> MTHHHHHHAMALTDRGMTYDLDPKDGSSAATKPVLEVTKKVFDTAADAAGQTVTVEFKVSGAEGKYATTGYHIYWDERLEVVATKTGAYAKKGAALEDSSLAKAENNGNGVFVAS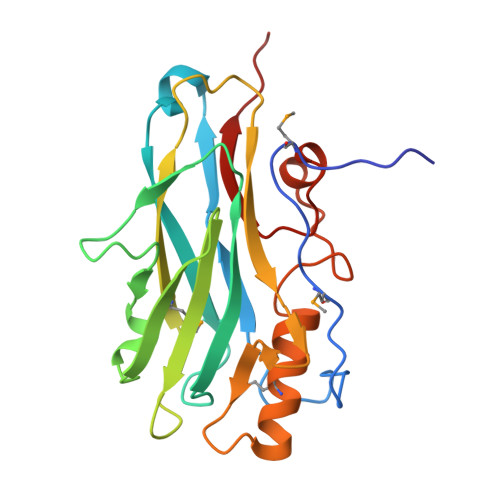GADDDFGADGVMWTVELKVPADAKAGDVYPIDVAYQWDPSKGDLFTDNKDSAQGKLMQAYFFTQGIKSSSNPSTDEYLVKANATYADGYIAIKAGEP> MALTQSVGGDSSADRLFPPQWICCDIRYLDVSILGKFAVVMADPPWDIHMELPYGTLTDDEMRRLNIPVLQDDGFLFLWVTGRAMELGRECLNLWGYERVDEIIWVKTNQLQRIIRTGRTGHWLNHGKEHCLVGVKGNPQGFNQGLDCDVIVAEVRSTSHKPDEIYGMIERLSPGTRKIELFGRPHNVQPNWITLGNQLDGIHLLDPDVVARFKQRYPDGIISKPKNL;> GLKGTQSLNPHNDYCQHFVDTGHRPQNFIRDVGLADRFEEYPKLRELIRLKDELIAKSNTPPMYLQADIEAFDIRELTPKFDVILLEPPLEEYYRETGITANEKCWTWDDIMKLEIDEIAAPRSFIFLWCGSGEGLDLGRVCLRKWGYRRCEDICWIKTNKNNPGKTKTLDPKAVFQRTKEHCLMGIKGTVKRSTDGDFIHANVDIDLIITEEPEIGNIEKPVEIFHIIEHFCLGRRRLHLFGRDSTIRPGWLTVGPTLTNSNYNAETYASYFSAPNSYLTGCTEEIERL

The complex of methyltransferase-like proteins 3 and 14 (METTL3-14) is the major enzyme that deposits N6-methyladenosine (m6A) modifications on messenger RNA (mRNA) in humans. METTL3-14 is the catalytic complex that transfers the methyl group from S-adenosylmethionine (SAM) to the substrate adenosine (Wang et al., 2016b; Wang et al., 2016a; Śledź and Jinek, 2016; Yoshida et al., 2022). The METTL3 MTase domain has the catalytically active SAM binding site and adopts a Rossmann fold that is characteristic of Class I SAM-dependent MTases. METTL14 plays a structural role for complex stabilisation and RNA binding.

In the METTL3-BA2 and -BA4 structures, the SAM moiety is superimposable with the METTL3-bound conformation of SAM, and adenosine is bound in the presumed catalytic site. A crystal structure with a BA representing the transition state of methyl transfer shows a direct involvement of the METTL3 side chains E481 and K513 in adenosine binding which is supported by mutational analysis. The METTL3-BA2 structure reveals that there can also be a hydrogen bond formed between D395 and the N6-atom of adenosine in the case of the non-alkylated RNA substrate. The BA2 structure further shows that adenosine is stabilised by additional hydrogen bonds from its N7- and O2’-atoms to the METTL3 side chains of E481 and K513, respectively. Taken together, adenosine swaps conformation from solvent exposed in the METTL3-BA4 structure to buried in the METTL3-BA2 structure where it forms hydrogen bonds with residues in the active site loop 2 (ASL2, METTL3 residues 507–515). The crystal structure of the complex with BA2 reveals a string of ionic interactions which involves charged side chains of METTL3 and the amino and carboxyl groups of the SAM analogue. The string consists of seven charged groups (four of which are positive): R536+ – SAM COO- – SAM NH3+ – D395- – K513+ – E481- – K459+. In BA2, the adenosine-N6 is situated, through the alkyl chain of the linker, at 1.9 Å away from the carbon corresponding to the Cε-atom of the methionine moiety in the SAM cofactor. Strikingly, the angle formed by the SAM-5’S – Cε – adenosine-N6 in METTL3 is 160.9° which is similar to the other MTases, and very close to the optimal 180° for an SN2 reaction in which the adenosine-N6 attacks the SAM-Cε and SAH becomes the leaving group. Hence, the adenosine of BA2 is in a suitable orientation for methyl transfer and BA2 represents a transition state mimic for METTL3.> GPGSEDLPLPPGWSVDWTMRGRKYYIDHNTNTTHWSHPLEREGLPPGWERVESSEFGTYYVDHTNKR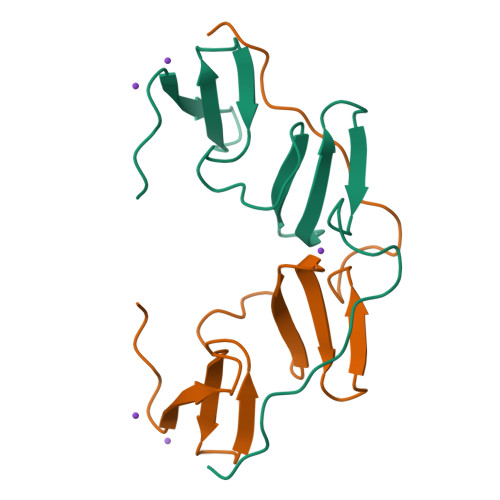AQYRHPCAPSVPPPYVAPPSYEG>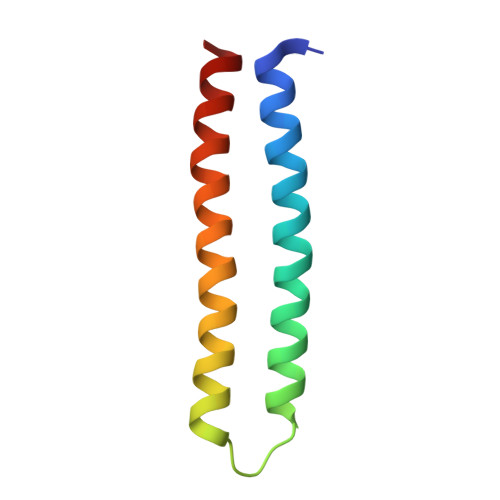 GSSPEEEKLKELLKELKKVLDRLKKILERNDEEIKKSDELDDESLLEDIVELLKEIIKLWKILVELSDILLKLIS> GSHMSLDINQIALHQLIKRDEQNLELVLRDSLLEPTETVV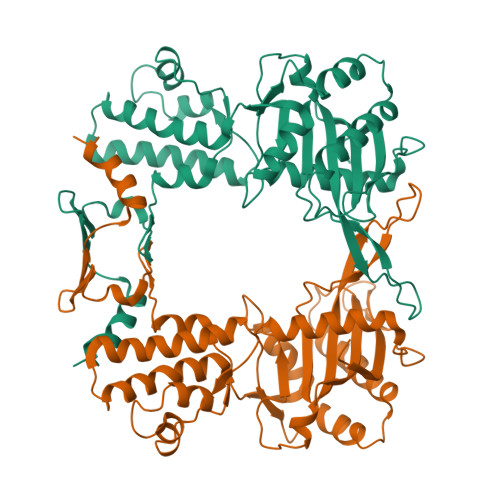EMVAELHRVYSAKNKAYGLFSEESELAQTLRLQRQGEEDFLAFSRAATGRLRDELAKYPFADGGFVLFCHYRYLAVEYLLVAVLSNLSSMRVNENLDINPTHYLDINHADIVARIDLTEWETNPESTRYLTFLKGRVGRKVADFFMDFLGASEGLNAKAQNRGLLQAVDDFTAEAQLDKAERQNVRQQVYSYCNEQLQAGEEIELKSLSKELAGVSEVSFTEFAAEKGYELEESFPADRSTLRQLTKFAGSGGGLTINFDAMLLGERIFWDPATDTLTIKGTPPNLRDQLQRRTSGGN>[8x]MHHHHHHTSKIEQPRWASKDSAAGAASTPDEKIVLEFVDALTSNDAAKLIEYFAEDTMYQNMPLPPAYGRDAVEQTLAGLFTVVSV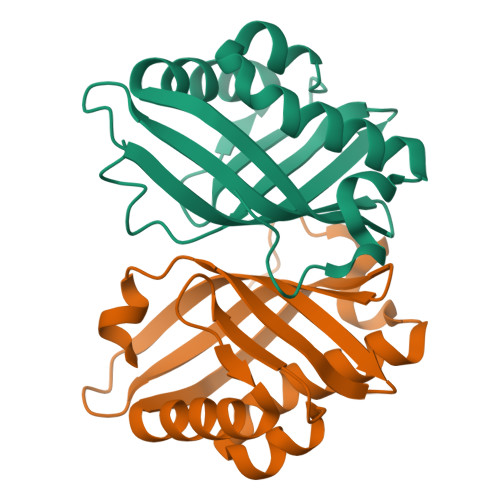DAVETFHIGSSNGLVYTERVDVLRALPTGKSYNFSILGVFQLTEGKITGWRDYFDLREFEEAVDLPLRG>MGRIKNKQFAVIGLGRFGGSICKELHRMGHEVLAVDINEEKVNAYASYATHAVIANATEENELLSLGIRNFEYVIVAIGANIQASTLTTLLLKELDIPNIWVKAQNYYHHKVLEKIGADRIIHPQKDMGVKIAQSLSDENVLNYIDLSDEYSIVELLATRKLD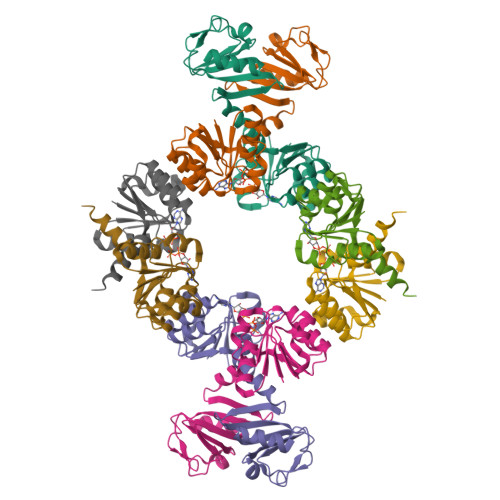SKSIIDLNVRAKYGCTILAIKHHGDICLSPAPEDIIREQDCLVIMGHKKDIKRFENEGM[8x]>[4x]GSDIPEHWEEDASWGPHRLAVLVPFRERFEELLVFVPHMRRFLSRKKIRHHIYVLNQVDHFRFNRAALINVGFLESSNSTDYIAMHDVDLLPLNEELDYGFPEAGPFHVASPELHPLYHYKTYVGGILLLSKQHYRLCNGMSNRFWGWGREDDEFYRRIKGAGLQLFRPSGITTGYKTFRHLHDPAWRKRDQKRIAAQKQEQFKVDREGGLNTVKYHVASRTALS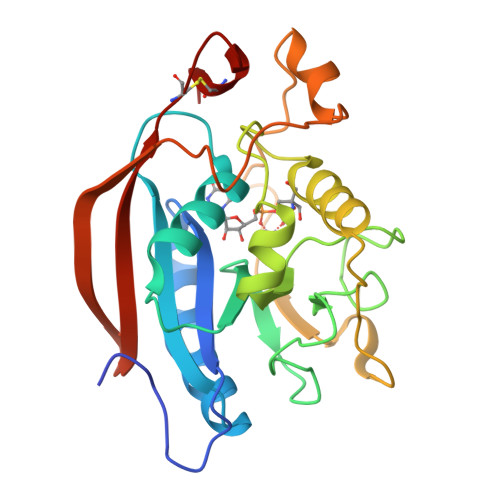VGGAPCTVLNIMLDCDKTATPWCTFS> MSDTKVYLLDGGSLVLDGYHVFWNRGPGGEVRFPVYSILI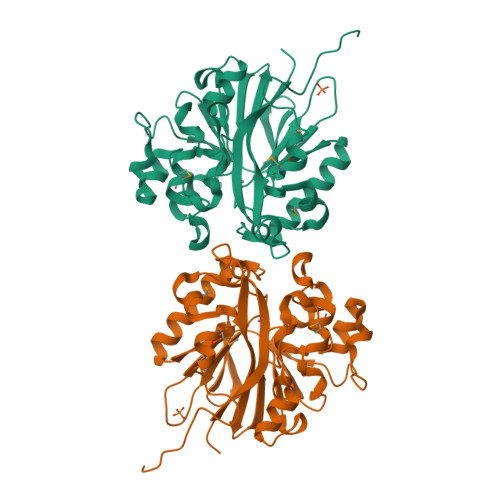EHAEGRFLIDTGYDYDHVMKVLPFEKPIQEKHQTIPGALGLLGLEPRDIDVVVNSHFHFDHCGGNKYFPHAKKICHRSEVPQACNPQPFEHLGYSDLSFSAEAAEARGATAQLLEGTTRANSTFEGIDGDVDLARGVKLISTPGHSIGHYSLLVEFPRRKPILFTIDAAYTQKSLETLCQAAFHIDPVAGVNSMRKVKKLAEDHGAELMYSHDMDNFKTYRTGTQFYGHHHHHH> SNAMFAPQGLAQFIKVNVTLENGEPVFIYTDANGQVCQGDITVTQAGTITYLLNDQTLKGLKFVGVGFVTPFDGIIDAVTISSDGMLVQLVDLDKTPGTTAFQFVLSNTANTLLVLSPD;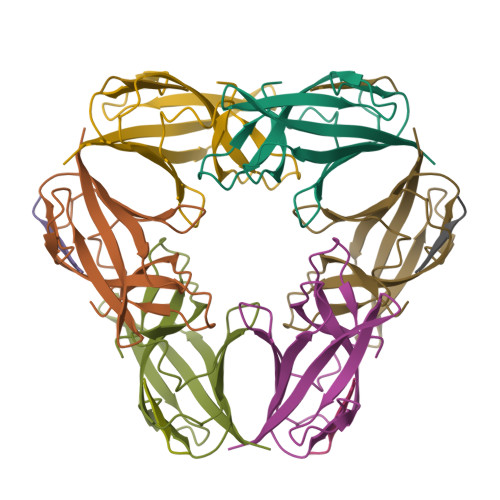> PQIINRPQN> GPLGSMASSNMKDETYYIALNMIQNYIIEYNTNKPRKSFVIDSISYDVLKAACKSVIKTNYNEFDIIISRNIDFNVIVTQVLEDKI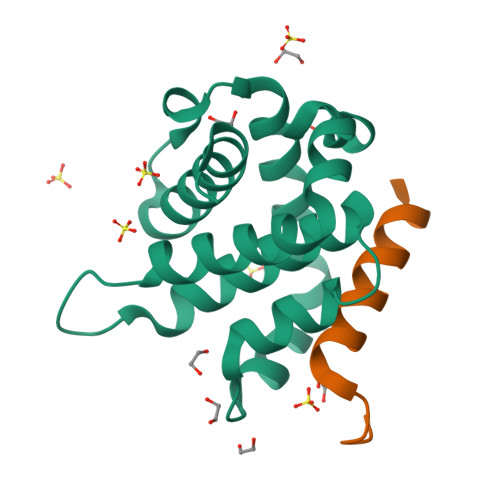NWGRIITIIAFCAYYSKKVKQDTSPQYYDGIISEAITDAILSKYRSWFIDQDYWNGIRIYKN;> ISSAIQVGHQLALIGDEFNRAYSRK(1R)-MENTHYL HEXYL PHOSPHONATE GROUP | C16 H33 O3 P | 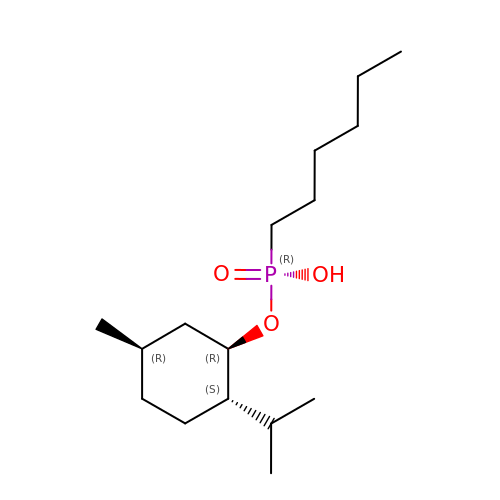WAVIZOVSJOXCKT-OWCLPIDISA-N> AQLRQFYVAAQGISWSYRPEPTNSSLNLSVTSFKKIVYREYEPYFKKEKPQSTISGLLGPTLYAEVGDIIKVHFKNKADKPLSIHPQGIRYSKLSEGASYLDHTFPAEKMDDAVAPGREYTYEWSISEDSGPTHDDPPCLTHIYYSHENLIEDFNSGLIGPLLICKKGTLTEGGTQKTFDKQIVLLFAVFDESKSWSQSSSLMYTVNGYVNGTMPDITVCAHDHISWHLLGMSSGPELFSIHFNGQVLEQNHHKVSAITLVSATSTTANMTVGPEGKWIISSLTPKHLQAGMQAYIDIKNCPKKTRNLKKITREQRRHMKRWEYFIAAEEVIWDYAPVIPANMDKKYRSQHLDNFS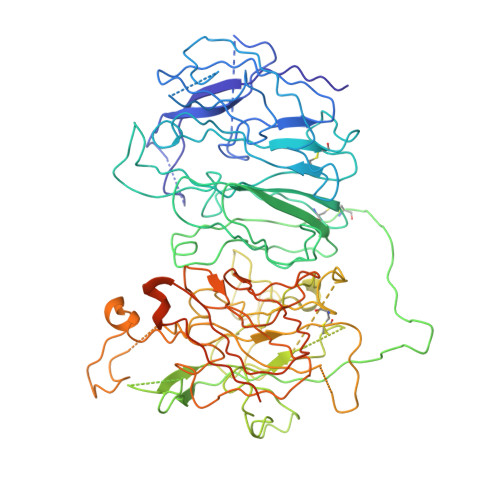NQIGKHYKKVMYTQYEDESFTKHTVNPNMKEDGILGPIIRAQVRDTLKIVFKNMASRPYSIYPHGVTFSPYEDEVNSSFTSGRNNTMIRAVQPGETYTYKWNILEFDEPTENDAQCLTRPYYSDVDIMRDIASGLIGLLLICKSRSLDRRGIQRAADIEQQAVFAVFDENKSWYLEDNINKFCENPDEVKRDDPKFYESNIMSTINGYVPESITTLGFCFDDTVQWHFCSVGTQNEILTIHFTGHSFIYGKRHEDTLTLFPMRGESVTVTMDNVGTWMLTSMNSSPRSKKLRLKFRDVKCIPDDDEDSYEIFEPPESTVMATRKMHDRLEPEDEESDADYDYQNRLAAALGIR>MAIAQLATEYVFSDFLLKEPTEPKFKGLRLELAVDKMVTCIAVGLPLLLISLAFAQEISIGTQISCFSPSSFSRDQAAFVDSYCWAAVQQKNSLQSESGNLPLWLHKFFPYILLLFAILLYLPPLFWRFAAAPHICSDLKFIMEELDKVYNRAIKAAKSARDLDMRDGACSVPGVTENLGQSLWEVSESHFKYPIVEQYLKTKKNSNNLIIKYISCRLLTLIIILLACIYLGYYFSLSSLSDEFVCSIKSGILRNDSTVPDQFQCKLIAVGIFQLLSVINLVVYVLLAPVVVYTLFVPFRQKTDVLKVYEILPTFDVLHFKSEGYNDLSLYNLFLEENISEVKSYKCLKVLENIKSSGQGIDPMLLLTNLGMIKMDVVDGKTPMSAEMREEQGNQTAELQGMNIDSETKANNGEKNARQRLLDSSCHHHHHHHH[7x]

Pannexins are single-membrane large-pore channels that release ions and ATP upon activation. Three isoforms of pannexins 1, 2, and 3, perform diverse cellular roles and differ in their pore lining residues. Pannexin protomers retain structural and topological similarity to innexins, connexins, and volume-regulated anion channels but remain as single-membrane channels and participate in ion-conductance and ATP release. The PANX isoforms, PANX1, PANX2, and PANX3 harbor substitutions in the residues that control channel gating and can have architectural differences that form the basis for altered properties among the three isoforms.

In order to observe if a dual substitution of both the residues (W74, R75) by charged amino acids could compensate for this behavior, we created a PANX1 double mutant (PANX1WR/RD) by substituting W74 and R75 with arginine and aspartate, respectively. Incidentally, these substitutions are similar to the pore residues of PANX2 revealed by multiple sequence alignment and structural comparison with PANX2. Surprisingly, we obtained a minor fraction of well-assembled PANX1WR/RD particles that allowed reconstruction of the PANX1WR/RD structure to a resolution of 3.2 Å. Whilst the global structure resembles the PANX1WT, the pore diameter was reduced to 9.3 Å compared to 12.1 Å in PANX1WT. The presence of R74 side chain facing the pore renders the pore of PANX1WR/RD highly cationic as compared to PANX1WT and the pore diameter resembles PANX2. The main interactions at the pore in PANX1WT are W74-R75 cation-pi interaction within the subunit and R75-D81 interaction between two subunits. As these residues were mutated, the interactions are lost in the PANX1WR/RD. Instead, in PANX1WR/RD, D75 of one protomer interacts with R74 of another protomer to stabilize the structure. We analyzed the differences of ATP-γS interactions with PANX1WR/RD and PANX1WT via MST binding. This revealed a reduced Kd value of 67 μM in PANX1WR/RD compared to ATP-γS binding affinity for PANX1WT (18 µM), suggesting that ATP interactions are moderately affected by these pore substitutions. The data revealed a two-fold reduction in current density in PANX1WR/RD compared to PANX1WT but retained an active channel despite the constriction of the pore radius.> GS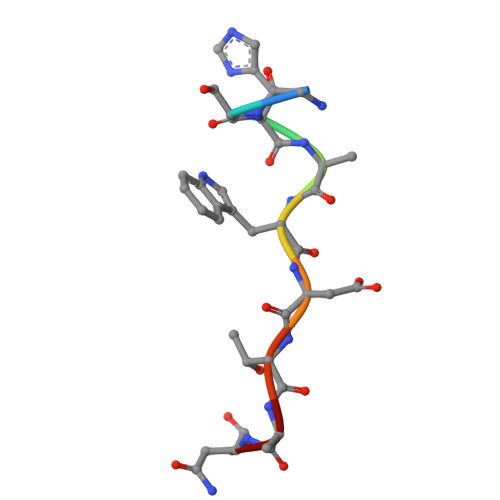HAWDTAN> AEKPLQV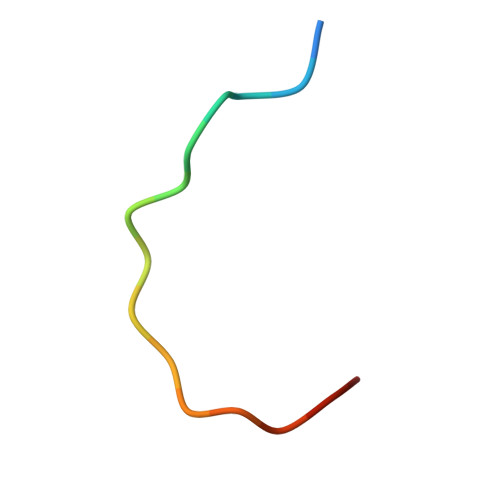AAVDSSVPRT>MSKSWGKFIEEEEAEMASRRNLMIVDGTNLGFRFKHNNSKKPFASSYVSTIQSLAKSYSARTTIVLGDKGKSVFRLEHLPEYKGNRDE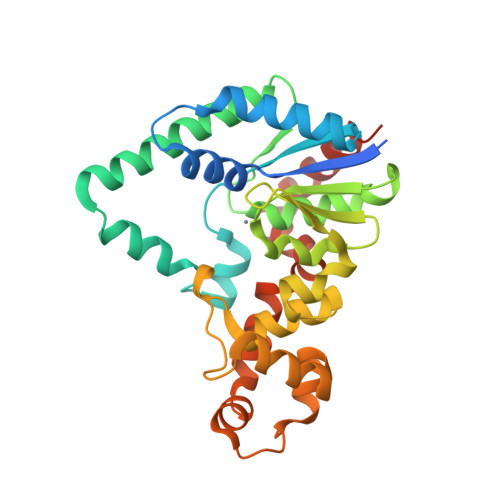KYAQRTEEEKALDEQFFEYLKDAFELCKTTFPTFTIRGVEADDMAAYIVKLIGHLYDHVWLISTDGDWDTLLTDKVSRFSFTTRREYHLRDMYEHHNVDDVEQFISLKAIMGDLGDNIRGVEGIGAKRGYNIIREFGNVLDIIDQLPLPGKQKYIQNLNASEELLFRNLILVDLPTYCVDAIAAVGQDVLDKFTKDILEIAEQ[2x]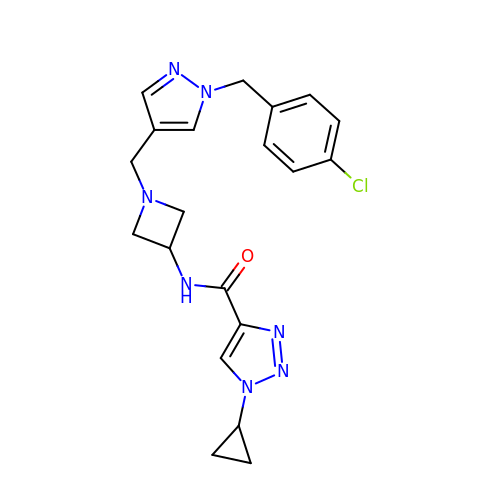N-[1-({1-[(4-chlorophenyl)methyl]-1H-pyrazol-4-yl}methyl)azetidin-3-yl]-1-cyclopropyl-1H-1,2,3-triazole-4-carboxamide | C20 H22 Cl N7 O | MOWCUCXGYVJUHU-UHFFFAOYSA-N>HHNKVRTCWNEGRPALAGWLQLPGTLHAEALARLDYDAVVIDMQHSPIDFGQVAPMLIAIELGGAEPFVRTQVNDPSDIMKLLDAGAYGIIAPMVNTRAEAQTLASALHYSPRGLRSFGPRRPSLRYGSGYLAQASETVVGLAMIETREALANIDEILSVDGIDGVFIGPTDLALDLGHAPLVDTEEAEVVSAIAHVRERAHAAGKRVGIFCGSGGFARVKLAEGFDFVTAAPDLAMLSAAARQVIADARAL[2x]

Here structural analysis of hydroxyketoacid aldolase from Sphingomonas wittichii RW1 (SwHKA) revealed a dynamic movement of the metal cofactor between two coordination spheres without protein scaffold rearrangements. Holo‐SwHKA forms a trimer of homodimers, in which each monomer adopts an (α/β)8 triosephosphate isomerase (TIM) barrel fold. In total, holo‐SwHKA contains six equivalent active sites; each of which is formed from amino acids from two different domain‐swapped dimers. The transition from M2+ R to M2+ A,S is induced by bidentate substrate binding and occurs without a concomitant rearrangement of the protein scaffold.

SwHKA displays activity both with Mn2+ and Mg2+. Crystals of WT apo‐SwHKA and mutant variants thereof were soaked with MgCl2 or MnCl2 to afford the holo‐enzyme. In the absence of substrates, M2+ R constitutes the predominant state and the M2+ A,W complex was observed with lower occupancy in crystal structures of holo‐SwHKA. Conversely, a square pyramidal coordination sphere at 2.4 Å distance from M2+ R constitutes the catalytically active state of holo‐SwHKA. Here, the coordination sphere no longer includes residue S116′, but only consists of E145, D171 next to three water molecules (M2+ A). The square‐pyramidal M2+ A,W complex was unanimously predicted for both Mg2+ and high‐spin Mn2+ in SwHKA to be lower in energy than the corresponding hypothetical octahedral M2+ A,W complex with four water ligands. Thermodynamics, therefore, favor a square‐pyramidal coordination geometry for M2+ A,W, which promotes substrate binding by providing a free coordination site. The energy difference between M2+ R and M2+ A,W in SwHKA therefore, seems to be substantially larger for protein‐metal complexes with Mg2+ than with Mn2+.>[6x]MNAQAEEFKKYLETNGIKPKQFHKKELIFNQWDPQEYCIFLYDGITKLTSISENGTIMNLQYYKGAFVIMSGFIDTETSVGYYNLEVISEQATAYVIKINELKEL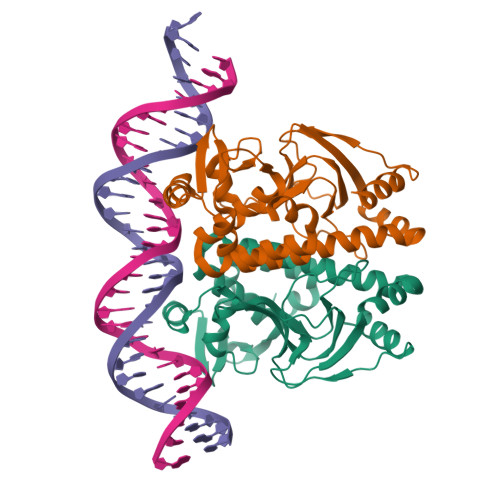LSKNLTHFFYVFQTLQKQVSYSLAKFNDFSINGKLGSICGQLLILTYVYGKETPDGIKITLDNLTMQELGYSSGIAHSSAVSRIISKLKQEKVIVYKNSCFYVQNLDYLKRYAPKLDEWFYLACPATWGKLN>[4x]SFELPALPYAK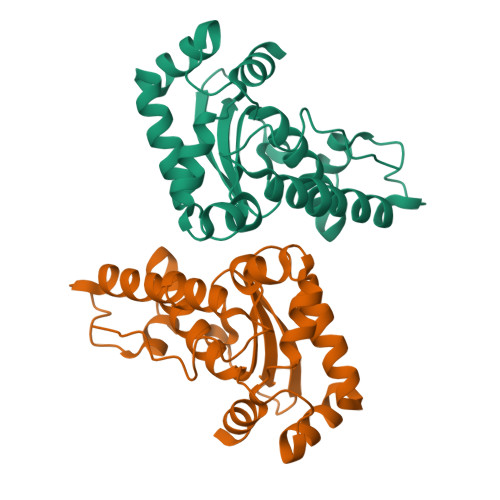DALAPHISAETIEYHYGKHHQTYVTNLNNLIKGTAFEGKSLEEIIRSSEGGVFNNAAEVWNHTFYWNCLAPNAGGEPTGKVAEAIAASFGSFADFKAQFTDAAIKNFGSGWTWLVKNSDGKLAIVSTSNAGTPLTTDATPLLTVDVWEHAYYIDYRNARPGYLEHFWALVNWEFVAKNLAA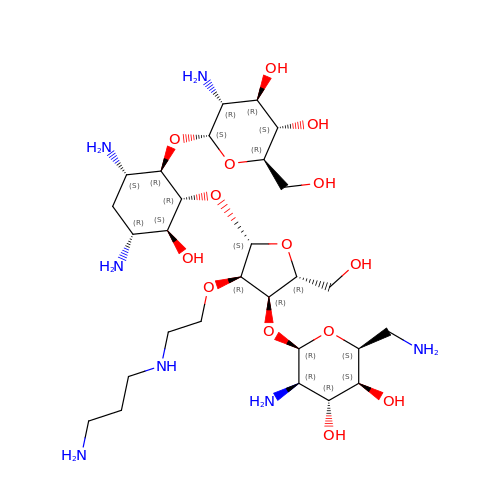(2S,3S,4R,5R,6R)-5-AMINO-2-(AMINOMETHYL)-6-((2R,3R,4R,5S)-4-(2-(3-AMINOPROPYLAMINO)ETHOXY)-5-((1R,2R,3S,5R,6S)-3,5-DIAMINO-2-((2S,3R,4R,5S,6R)-3-AMINO-4,5-DIHYDROXY-6-(HYDROXYMETHYL)-TETRAHYDRO-2H-PYRAN-2-YLOXY)-6-HYDROXYCYCLOHEXYLOXY)-2-(HYDROXYMETHYL)-TETRAHYDROFURAN-3-YLOXY)-TETRAHYDRO-2H-PYRAN-3,4-DIOL | C28 H57 N7 O14 | FJVLHNJZMYGVLT-XXJRHLBLSA-N>ASWSHPQFEKIEGRRDRGPEFMAKQYKNLVNGEWKLSENEITIYAPATGEELGSVPAMTQAEVDAVYASAKKALSDWRTLSYVERAAYLHKAADILVRDAEKIGAILSKEVAKGHKAAVSEVIRTAEIINYAAEEGLRMEGEVLEGGSFEAASKKKIAIVRREPVGLVLAISPFNYPVNLAGSKIAPALIAGNVVALKPPTQGSISGLLLAEAFAEAGIPAGVFNTITGRGSVIGDYIVEHEAVNFINFTGSTPIGEGIGKLAGMRPIMLELGGKDSAIVLEDADLALAAKNIVAGAFGYSGQRCTAVKRVLVMDKVADQLAAEIKTLVEKLSVGMPEDDADITPLIDTSAADFVEGLIKDATDKGATALTAFNREGNLISPVLFDHVTTDMRLAWEEPFGPVLPIIRVTTVEEAIKISNESEYGLQASIFTTNFPKAFGIAEQLEVGTVHLNNKTQRGTDNFPFLGAKKSGAGVQGVKYSIEAMTTVKSVVFDIQ[8x]

GapN catalyzes the irreversible oxidation of glyceraldehyde 3-phosphate (G3P) to 3-phosphoglycerate (3-PG) while reducing NADP+ to NADPH. As S. pyogenes lacks the oxidative part of the pentose phosphate pathway, GapN appears to be the major NADPH source for the bacterium. The GapN-monomer from S. pyogenes, like its counterparts from other organisms can be subdivided into three domains (Cobessi et al., 1999). The monomers assemble into a tetramer displaying D2 symmetry which is formed by two interlacing dimers with dimer-dimer contacts primarily mediated by the protruding domain, while contacts within each dimer are formed by a β-sheet of the protruding domain interacting with a β-sheet of the catalytic α/β domain via salt bridges as well as α-helices (residues 232–251) of the Rossmannoid fold of each chain.

To further characterize the function of the S. pyogenes GapN and provide a starting point for future screening campaigns, we determined the crystal structure of the GapN by molecular replacement using the apo-form of an S. mutans tetramer as a search model. The structure revealed a covalent modification of the enzyme at the active site residue C284, which could be modeled as β-mercaptoethanol although this compound was not present during purification. Hence, the enzyme must have been modified following heterologous expression in E. coli. Determination of the crystal structure of the S. pyogenes GapN apo-enzyme revealed an unusual cis-peptide in proximity to the catalytic binding site. In all chains of the wild-type and C284S variant a cis-peptide was observed while only half of the chains in the reference structure from S. mutans were modeled in the cis configuration. Considering that the formation of a cis-peptide outside an X-P (X denoting any amino acid) peptide is rather rare, the electron density maps of our structures and the published structures were critically examined. This analysis confirmed the formation of a cis-peptide bond in both S. pyogenes as well as in S. mutans. As this peptide bond is within 11.2 Å of the active site, it might be relevant for the proper function of the enzyme.> AADPLGQALRAIG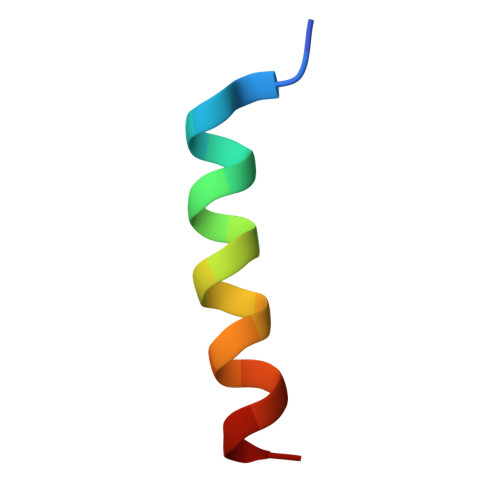DEFETRFR> GEVNKKDVKIETNTNKKDSEKENVNNTQENVSVEKQSAKKAKVKE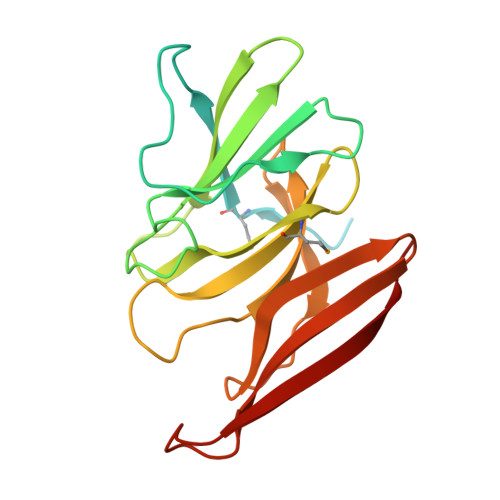DNSKKMFLKKELGKNSKPTFATKWKNSSNNKFSACIEGKGENALEEGVGKIYIKNLKEQSKWELDLDQDQQKNTPKYIDWFDDNNLMVVISRAHGTVSQGGILYKVNIETGQATELYNTKDNKKQVVYAVKKGDKIDVQILVYEDDDLLESHEETKTITVK>[3x]ADPTEPSSPPGAPSQPVVTEITKNSITLTWKPNPQTGAAVTSYVIEAFSPAAGNTWRTVADGVQLETHTVSGLQPNTIYLFLVRAVGAWGLSEPSPVSEPVRTQDSEFHHHHHH;>ADPRGHNFCAEGPKCGENSECKNWNTKATCECKSGYISVQGDSAYCEDIDECAAKMHYCHANTVCVN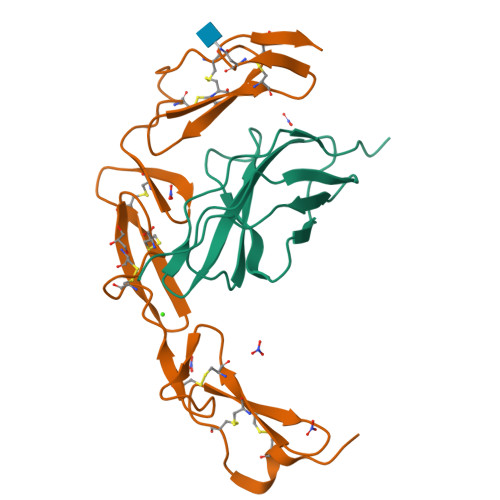LPGLYRCDCVPGYIRVDDFSCTEHDECGSGQHNCDENAICTNTVQGHSCTCKPGYVGNGTICRAEFHHHHHH[3x]> MHLNPAEKEKLQIFLASELALKR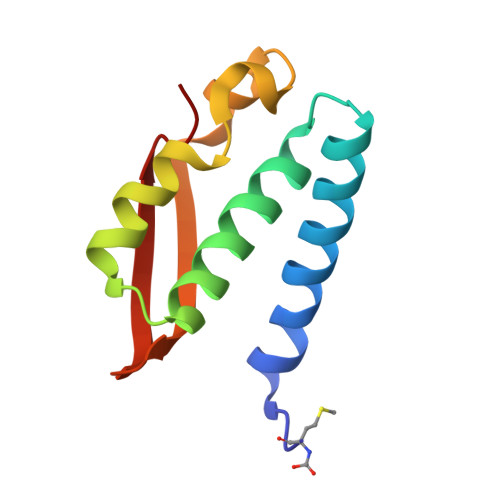KARGLKLNYPEAVAIITSFIMEGARDGKTVAMLMEEGKHVLTRDDVMEGVPEMIDDIQAEATFPDGTKLVTVHNPIS>SNAMKDFHFDAISAFENYEIEKMRDGHVVVTTKVVNSSLNYYGNAHGGYLFTLCDQISGLVVISLGLDGVTLQSSINYLKAGKLDDVLTIKGECVHQGRTTCVMDVDITNQEGRNVCKATFT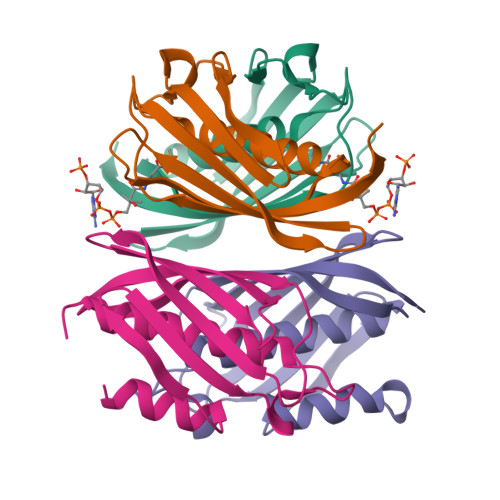MFVTGQRSEERRVRI[8x]4-AMINO-2-DEOXY-2,3-DEHYDRO-N-ACETYL-NEURAMINIC 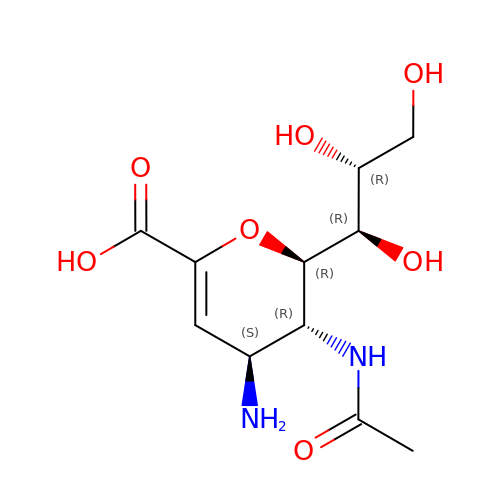ACID | C11 H18 N2 O7 | NKENBBIXEGPQLS-UFGQHTETSA-N>[6x]LKKLCKL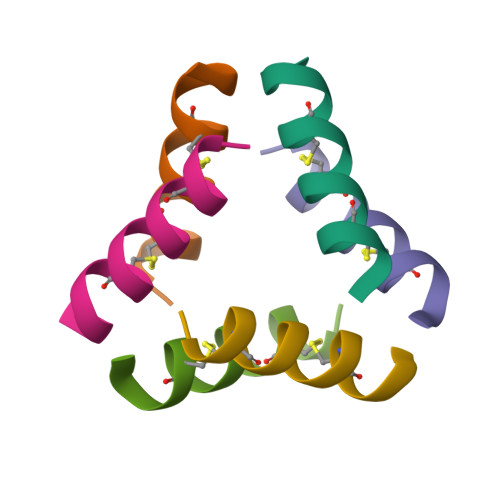LKKLCKLAG>EQKTRPFTLPNLPLSSLSNSRAPLPISSMGISPDNVQSVQFQNGRCTLDGRLVGTTPVSLSHVAKIRGTSNGTVINLTELDGTPFHPFEGPAPIGFPDLGGCDWHINMTQFGHSSQTQYDVDTTPDTFVPHLGSIQANGIGSGNYVGVLSWISPPSHPSGSQVDLWKIPNYGSSITEATHLAPSVYPPGFGEVLVFFMSKMPGPGAYNLPCLLPQEYISHLASEQAPTIGEAALLHYVDPDTGRNLGEFKAYPDGFLTCVPNGASSGPQQL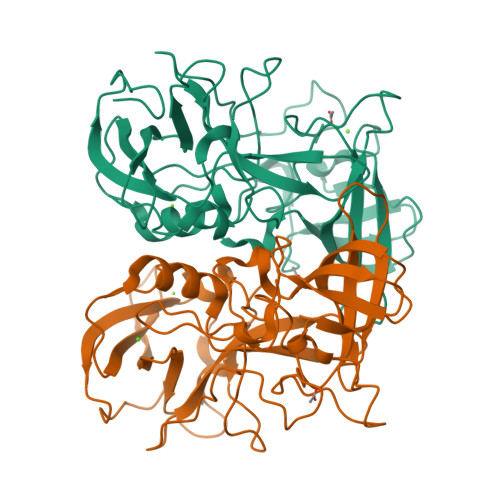PINGVFVFVSWVSRFYQLKPVGTV[2x]>[6x]GHMATIHPTAIVDEGARIGAHSRIWHWVHICGGAEIGEGCSLGQNVFVGNRVRIGNRVKIQNNVSVYDNVFLEDDVFCGPSMVFTNVYNPRAAIERKSEYRDT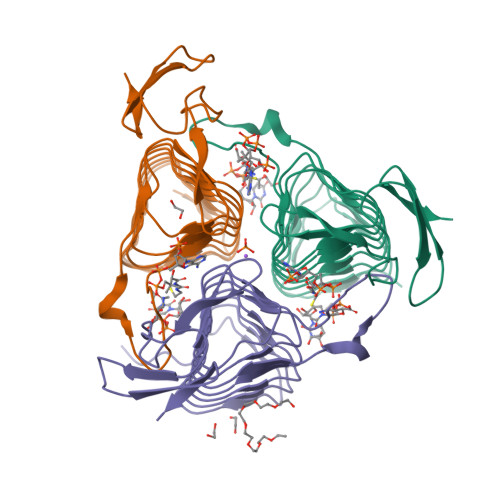IVRQGATLGANCTVVCGATIGRYAFVGAGAVVNKDVPDFALVVGVPARQIGWMSRHGEQLDLPLRGNAEATCPHTGERYILTDGVCRLA> FHLTTRNGEPHMIVSRQEKGKSLLFKTEDGVNMCTLMAMDLGELCEDTITYKCPLLRQNEPED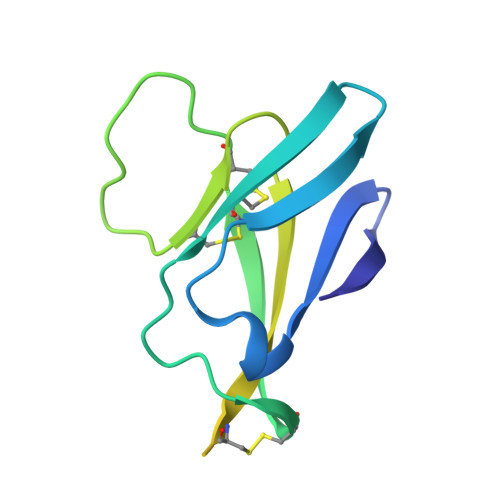IDCWCNSTSTWVTYGTCTTMGEHSTEKSSVALVPHVGMGLETRTETWMSSEGAWKHVQRIETWILRH>[3x]MMITLRKLPLAVAVAAGVMSAQAMAMACAGGGSTPLPLPQQQPPQQEPPPPPVPLASRAACEALKDGNGDMVWPNAATVVEVAAWRDAAPATASAAALPEHCEVSGAIAKRTGIDGYPYEIKFRLRMPAEWNGRFFMEGGSGTNGSLSAATGSIGGGQIASALSRNFATIATDGGHDNAVNDNPDALGTVAFGLDPQARLDMGYNSYDQVTQAGKAAVARFYGRAADKSYFIGCSEGGREGMMLSQRFPSHYDGIVAGAPGYQLPKAGISGAWTTQSLAPAAVGLDAQGVPLINKSFSDADLHLLSQAILGTCDALDGLADGIVDNYRACQAAFDPATAANPANGQALQCVGAKTADCLSPVQVTAIKRAMAGPVNSAGTPLYNRWAWDAGMSGLSG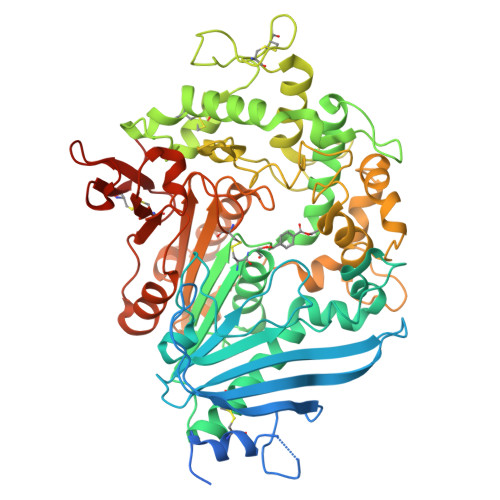TTYNQGWRSWWLGSFNSSANNAQRVSGFSARSWLVDFATPPEPMPMTQVAARMMKFDFDIDPLKIWATSGQFTQSSMDWHGATSTDLAAFRDRGGKMILYHGMSDAAFSALDTADYYERLGAAMPGAAGFARLFLVPGMNHCSGGPGTDRFDMLTPLVAWVERGEAPDQISAWSGTPGYFGVAARTRPLCPYPQIARYKGSGDINTEANFACAAPPLEHHHHHH>[4x]MKKLTSGPALPGKLADCTAQDLNRTELFLVEGDSAGGSAKQARDREYQAIMPLKGKILNTWEVSSDEVLASQEVHDISVAIGIDPDSDDLSQLRYGKICILADADSDGLHIATLLCALFVRHFRTLVKEGHVYVALPPLYRIDLGKEVYYALTEEEKTGVLEQLKRKKGKPNVQRFKGLGEMNPMQLRETTLDPNTRRLVQLVISDEDEQQTTAIMDMLLAKKRSEDRRNWLQEKGDMADLEVEFMSDMAERLALHEFTENAYLNYSMYVIMDRALPFIGDGLKPVQRRIVYAMSELGLNASAKFKKSARTVGDVLGKYHPHGDSACYEAMVLMAQPFSYRYPLGDGQGNWGAPDDPKSFAAMRYTESRLSKYAELLLSELGQGTVDWVPNFDGTLQEPKMLPARLPNILLNGTTGIAVGMATDIPPHNLREVAKAAITLIEQPKTTLDELLDIVQGPDFPTEAEIITSRAEIRKIYQNGRGSVRMRAVWSKEDGAVVITALPHQVSGAKVLEQIAAQMRNKKLPMVDDLRDESDHENPTRLVIVPRSNRVDMEQVMNHLFATTDLEKSYRINLNMIGLDGRPAVKNLLEILSEWLVFRRDTVRRRLNHRLEKVLKRLHILEGLLVAFLNIDEVIEIIRTEDEPKPALMSRFGISETQAEAILELKLRHLAKLEEMKIRGEQSELEKERDQLQAILASERKMNNLLKKELQADADAFGDDRRSPLHEREEAKAMSHHHHHH

In bacteria, topoisomerase IV, a tetramer of two ParC and two ParE subunits, unlinks daughter chromosomes prior to cell division, whereas the related enzyme gyrase, a GyrA2GyrB2 tetramer, supercoils DNA and helps unwind DNA at replication forks. Both enzymes act via a double-strand DNA break involving a cleavage complex and are targets for quinolone antimicrobials that act by trapping these enzymes at the DNA-cleavage stage and preventing strand re-joining. Levofloxacin is a broad-spectrum third-generation fluoro­quinolone antibiotic. It is active against Gram-positive and Gram-negative bacteria and functions by inhibiting gyrase and topoisomerase IV.

We have co-crystallized the K. pneumoniae topoisomerase IV ParC/ParE breakage-reunion domain (ParC55; residues 1–490) and ParE TOPRIM domain (ParE30; residues 390–631) with a precut 34 bp DNA duplex (the E-site), stabilized by levofloxacin. The X-ray crystal structure of the complex was determined to 3.35 Å resolution, revealing a closed ParC55 dimer flanked by two ParE30 monomers. Residues 6–30 of the N-terminal α-helix α1 of the ParC subunit again embrace the ParE subunit, ‘hugging’ the ParE subunits close to either side of the ParC dimer. In contrast, the K. pneumoniae complex was formed by co-crystallizing the topoisomerase tetramer complex in the presence of a 34-base-pair pre-cleaved DNA in the presence of levofloxacin. The methylpiperazine at C7 (using the conventional quinolone numbering; C9 in the IUPAC numbering) on the drug extends towards residues Glu474 and Glu475 for S. pneumoniae and towards Gln460 and Glu461 for K. pneumoniae, where the glutamate at 474 is substituted by a glutamine at 460 in the Klebsiella strain. Interestingly, for S. pneumoniae we observe only one possible orientation of the C7 groups in both sub­units, while for K. pneumoniae we can see two: one with the same orientation as in S. pneumoniae and other rotated 180° away. They both exist within the same crystal in the two different dimers in the asymmetric unit. For K. pneumoniae both of the carboxyl O atoms are pointing towards the Mg2+ ion at distances of 4.86 and 4.23 Å. The CC25 (the drug concentration that converted 25% of the supercoiled DNA substrate to a linear form) was 0.5 µM for the Klebsiella enzyme and 1 µM for the pneumococcal enzyme.>MTVLATSRLHIEGDFRGYGSLDKSPPGALETLNRLMQNNHDEFDMFWRPDAGHNHTAHSLLSVYALGGSSADLERAYRDDDPHQVPIGAVDHSVVASLKDPRIFIHRMQRLDQYSNYLRFFEERIEARGWKAVVVEYLFSRSDAAEAMLGQLFEGAYHPLIQLGFGIEFELPGLVAEGLAHCAAHDAANIIPFFQKAEKLAKSGSVAPAPLVELYKEVRDTEKIRLAAKMTQGPVRVRDGVMGEAQDDIAAVAAKFQVGPDGLKQAIIETTSCAAYSCGGAQRPGKVAKVDFFFMHMVVSSIFLSILARQDWLETEDKIRLVEWKGRLDLVWYAASSAPALDRKWLEQYQPTLSAGMDWRALYRAVTVEPDDGHLAKIVRSLKWAEEEAKGVETSETIPVAGSG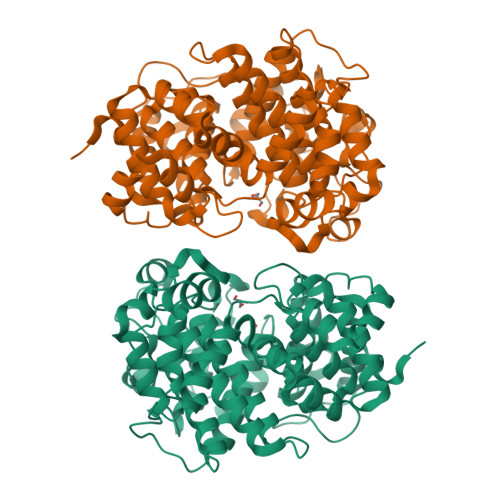WFKLAQMAYDSTAHLPIPAKWIMGAGYDFLWTRVDSLPAA[2x]> MKRKPNSNQNNNNNRGNGNGLRRVRGGRVSRRRVVINQSNQSMPVTSNGAPLQALTSYSRPNVNKISRLGPDSDFLTSVVAKASTSIVTPADRILVKQPLSASSFPGTRITGLSSYWERYKWLSAVARYVPAVPNTVACQFVMYIDTDPLDDPSNISDDNQIVRQAVSQAGSNQFNFNTSKTVPLIVRADNQYYYTGVDKQNLRFSLQGILYIIQVTDLINFNGELITQDLTCGSLFLDWLVNFSIPQINPTSLTDVRVDKAVNFIKPEVSGVAEIQTVTGLSPSTSYLLTPAFLEQNFQSEAGIYILSATPVEGEGTISINMDPTVTTVSGFIKVKTDTFGTFDLSVVLTTASKKQTTGFNIIAATS

A major factor that limits the expansion of shrimp cultures is, however, infectious diseases from viruses, such as P. vannamei nodavirus (PvNV) and M. rosenbergii nodavirus (MrNV), which have inflicted heavy economic losses. The Nodaviridae genome comprises two single-stranded positive-sense RNA that encode the capsid protein for viral capsid assembly, the RNA polymerase for RNA replication, and the B2 protein for host RNA interference suppressor. While the shell domains (S-domains) of PvNV and MrNV contain conserved sequences of 62% identity, the protrusion domains (P-domains) and N-arms show low sequence identities of only 17% and 43%, respectively. In this work, we have determined the cryo-EM structures of T = 3 and T = 1 PvNV-LPs at atomic resolution, the crystal structures of the P-domains of PvNV and MrNV (PvNVPd and MrNVPd), and the crystal structure of the S-domain of PvNV (ΔN-ARM-PvNVSd) in the T = 1 subviral particle (SVP).

The structure of a smaller-sized T = 1 PvNV-LP particle was determined by cryo-EM at 3.7 Å resolution. The subunit A of the T = 3 PvNV-LP was used to assist in the building of a complete model for the T = 1 PvNV-LP. The final atomic model of a capsid protein in the T = 1 PvNV-LP includes residues 64–368 without the mostly structurally disordered N-terminal region (residues 1–63), and comprises a canonical viral jelly-roll S-domain with two four-stranded antiparallel β-sheets (BIDG and CHEF), a linker and a P-domain. Totally, 60 PvNV capsid proteins were structurally equivalent with the I2, I3, and I5 axes. A structural comparison of one subunit of T = 1 PvNV-LP and the subunit A of T = 3 PvNV-LP reveals RMSD < 0.2 Å. The 30 spikes on the outer surface are also readily discernible. They might be mainly involved in the homo-dimeric capsomere interactions, resulting in the A/A dimer with a bent conformation with angle ~144°, similar to the A/B dimer of T = 3 PvNV-LP. Although there is no extra density at the interface between two neighboring subunits of the T = 1 PvNV-LP, the high structural homology of the S-domains in the T = 3 and T = 1 PvNV-LPs suggests that the Ca2+-binding site is conserved. The T = 3 and T = 1 PvNV-LPs have the similar structures of the S-domain, linker, and P-domain, but the N-ARM and N-arm of T = 1 PvNV-LP are more flexible. In contrast with the T = 3 PvNV-LP, T = 1 PvNV-LP, with only A/A dimers, has a bent conformation and a smaller inner cavity, and would associate weakly with the RNA nucleotide, rendering free or partial viral genome encapsidation.>GHHHHHHVPAFLSKLWTLVEETHTNEFITWSQNGQSFLVLDEQRFAKEILPKYFKHNNMASFVRQLNMYGF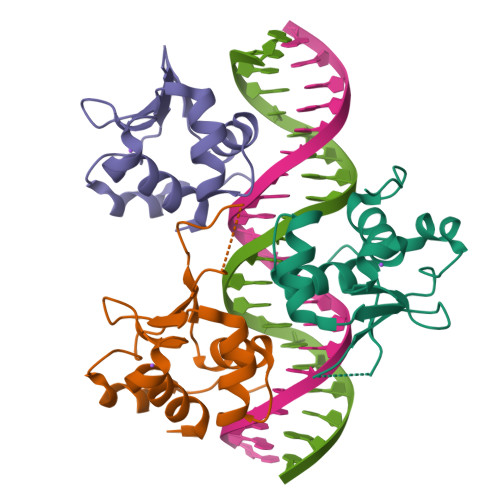RKVVHIDSGIVKQERDGPVEFQHPYFKQGQDDLLENIKRKVS[3x]>GPGSMKVEKVFFVTSPIYYVNAAPHIGHVYSTLITDVIGRYHRVKGERVFALTGTDEHGQKVAEAAKQKQVSPYDFTTAVAGEFKKCFEQMDYSIDYFIRTTNEQHKAVVKELWTKLEQKGDIYLGRYEGWYSISDESFLTPQNITDGVDKDGNPCKVSLESGHVVTWVSEENYMFRLSAFRERLLEWYHANPGCIVPEFRRREVIRAVEKGLPDLSVSRARATLHNWAIPVPGNPDHCVYVWLDALTNYLTGSRLRVDESGKEVSLVDDFNELERFPADVHVIGKDILKFHAIYWPAFLLSAGLPLPKKIVAHGWWTKDRKKISKSLGNVFDPVEKAEEFGYDALKYFLLRESGFSDDGDYSDKNMIARLNGELADTLGNLVMRCTSAKINVNGEWPSPAAYTEEDESLIQLIKDLPGTADHYYLIPDIQKAIIAVFDVLRAINAYVTDMAPWKLVKTDPERLRTVLYITLEGVRVTTLLLSPILPRKSVVIFDMLGVPEVHRKGIENFEFGAVPPGTRLGPAVEGEVLFS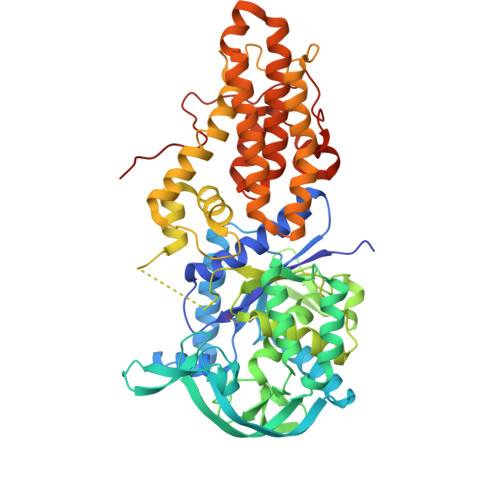KRSTENTKST[2x]> SMPPIFLPPPNYLFVRDVWKSNLYSEFAVIRQLVSQYNHVSISTEFVGTLARPIGTFRSKVDYHYQTMRANVDFLNPIQLGLSLSDANGNKPDNGPSTWQFNFEFDPKKEIMSTESLELLRK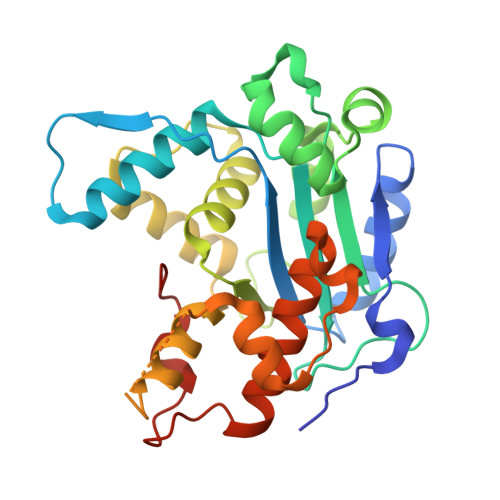SGINFEKHENLGIDVFEFSQLLMDSGLMMDDSVTWITYHAAYDLGFLINILMNDSMPNNKEDFEWWVHQYMPNFYDLNLVYKIIQEFKNPQLQQSSQQQQQQQYSLTTLADELGLPRFSIFTTTGGQSLLMLLSFCQLSKLSMHKFPNGTDFAKYQGVIYGIDGDQ>[2x]MGSSHHHHHHSSLVPRGSHMASQSMITPTTQIAGAGVLGNDRKPDESCARAAAAADPGPPTRPAHNAAGVSPEMVQVPAEAQRIVVLSGDQLDALCALGLQSRIVAAALPNSSSSQPSYLGTTVHDLPGVGTRSAPDLR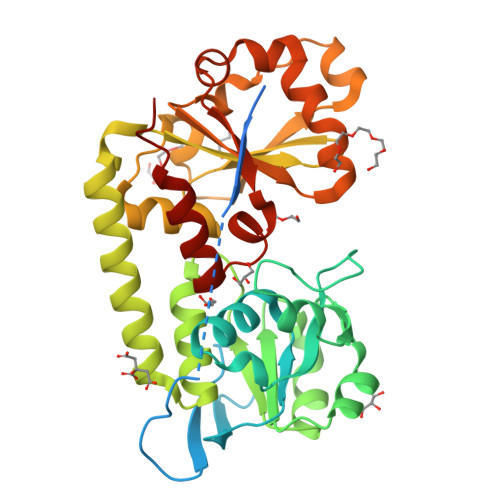AIAAAHPDLILGSQGLTPQLYPQLAAIAPTVFTAAPGADWENNLRGVGAATARIAAVDALITGFAEHATQVGTKHDATHFQASIVQLTANTMRVYGANNFPASVLSAVGVDRPPSQRFTDKAYIEIGTTAADLAKSPDFSAADADIVYLSCASEAAAERAAVILDSDPWRKLSANRDNRVFVVNDQVWQTGEGMVAARGIVDDLRWVDAPIN2-[(1-methyl-1H-benzimidazol-2-yl)methyl]-6-morpholin-4-ylpyrimidin-4(3H)-one | C17 H19 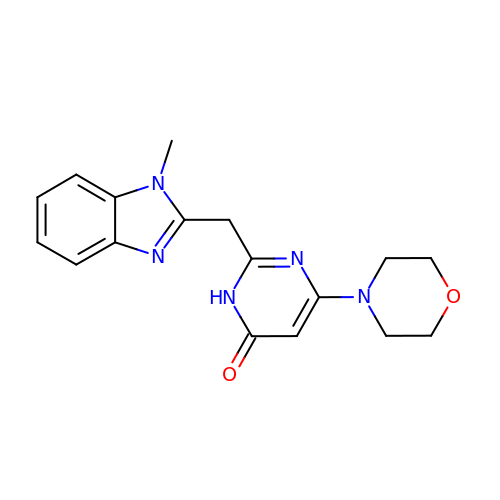N5 O2 | XLESLWHDVUIEMT-UHFFFAOYSA-N Here we describe a new mechanism by which foot-and-mouth disease virus (FMDV) can become resistant to ribavirin. Amino acid changes in the viral polymerase, selected by ribavirin, are able to modify the types of mutations produced in the presence of ribavirin. P44S but not P169S was detected in a 70% proportion in R-Ap35, as evidenced by analysis of both the consensus sequences and their corresponding mutant spectra. These results suggest that the three substitutions in 3D were selected sequentially during replication in the presence of increasing concentrations of R: first M296I, then P44S and finally P169S. To identify possible structural modifications of the viral polymerase associated with the important alterations of the mutational spectrum in progeny RNA, and to investigate how these modifications can affect RNA binding and polymerase activity, the different mutant 3Ds were incubated with the heteropolymeric sym/sub-U RNA of sequence 5′GCAUGGGCCC3′, crystallized, and analyzed by X-ray diffraction.

Since the biochemical results indicate that P44S plays a critical role in the misincorporation of RMP into RNA by 3D, and a 3D(P44S)-RNA complex was not obtained, we attempted the crystallization of the double mutant 3D(P44S, M296I) in complex with RNA. 3D(P44S, M296I) also crystallized in the space group P3221 space group, with the sym/sub-U RNA incorporated in the structure. The analysis of the electron density showed also the presence of the duplex portion of the template-primer RNA in the central channel of the polymerase of the trigonal 3D(P44S, M296I) and 3D(SSI) crystals. In addition, two of the four nucleotides of the 5′ overhang moiety (A3 and U4) were reasonably well defined, occupying the template channel, in both structures. The conformation and interactions of loop β9-α11 are identical in the 3D(P44S, M296I) and 3D(SSI) complexes, retaining the same structure that was previously observed in 3D (M296I) in complex with RNA. In 3D(P44S, M296I)-RNA and 3D(SSI)-RNA complexes the re-oriented residue R17 points to the polymerase interior, interacting with the side chain of residues N41 (which lies in the same loop of the substituted amino acid S44), and with Y285. Nucleotide A3 appears also reoriented, flipped-out towards a pocket formed by amino acids M16, P117, G118, Q160, F162, V181 and V183. These structural results indicate that the small movements in the loop, that contains the substituted residue S44, facilitate the large conformation changes of the 3D N-terminal residues M16-K18, and the reorientation of the template nucleotide A3. The conformational changes in the main and side chains of residues M16 and R17 allow the opening of a hydrophobic pocket formed by residues of motifs G and F and by M16 that facilitates the entrance of nucleotide A3. The polymerase with substitution M296I that acquired substitution P44S maintained the alteration of loop β9-α11 previously described for 3D (M296I).

> GLIVDTRDVEERVHVMRKTKLAPTVAHGVFNPEFGPAALSNKDSRLNEGVVLDEVIFSKHKGDTKMSAEDKALFRRCAADYASRLHSVLGTANAPLSIYEAIKGVDGLDAMEPDTAPGLPWALQGKRRGALIDFENGTVGPEVEAALKLMEKREYKFACQTFLKDEIRPMEKVRAGKTRIVDVLPVEHILYTRMMIGRFCAQMHSNNGPQIGSAVGCNPDVDWQRFGTHFAQYRNVWDVDYSAFDANHCSDAMNIMFEEVFRTEFGFHPNAEWILKTLVNTEHAYENKRITVEGGIPSGCSATSIINTILNNIYVLYALRRHYEGVELDTYTMISYGDDIVVASDYDLDFEALKPHFKSLGQTITPADKSDKGFVLGHSITDVTFLKRHFHMDYGTGFYKPVMASKTLEAILSFARRGTIQEKLISVAGLAVHSGPDEYRRLFEPFQGLFEIPSYRSLYLRWVNAVCGDAAALAH3-(6-ethoxynaphthalen-2-yl)-1-(piperidin-4-ylmethyl)-1H-pyrazolo[3,4-d]pyrimidin-4-amine | C23 H26 N6 O | 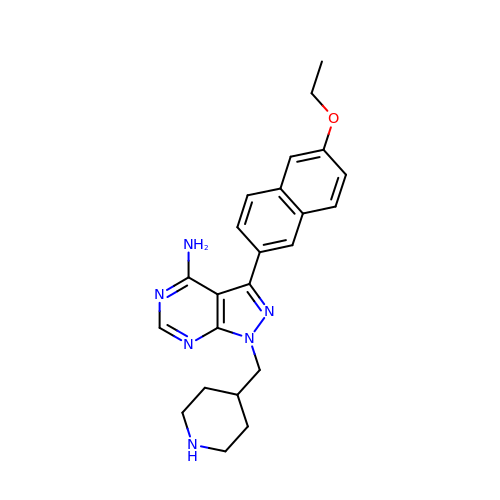DLMBMHOJKBPKLK-UHFFFAOYSA-N> MDFYQLPGSPPCRAVALTAAALDIEMNFKQVNLMNGEHLKPEFLKINPQHTIPTIDDNGFRLWESRAIMTYLADQYGKNDTLYPKDLKKRAIVNQRLYFDMCSLYKSFMDYYYPIIFMKAVKDQAKYENIGTALSFLDKFLEGENYVAGKNMTLADLSIVSTVSTLEALDYDLSKYKN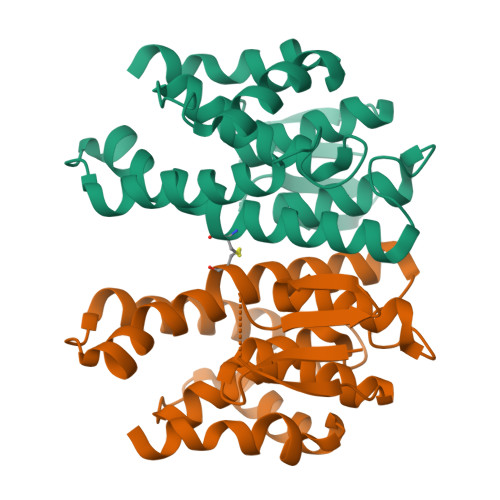VTRWFAKIKPEIPKYEEYNNAGLKMFKELVNEKLSKK>MILSDKDIIDYVTSKRIIIKPFNKDFVGPCSYDVTLGDEFIIYDDEVYDLSKELNYKRIKIKNSILVCPLNYNLTEEKINYFKEKYNVDYVVEGGVLGTTNEYIELPNDISAQYQGRSSLGRVFLTSHQTAG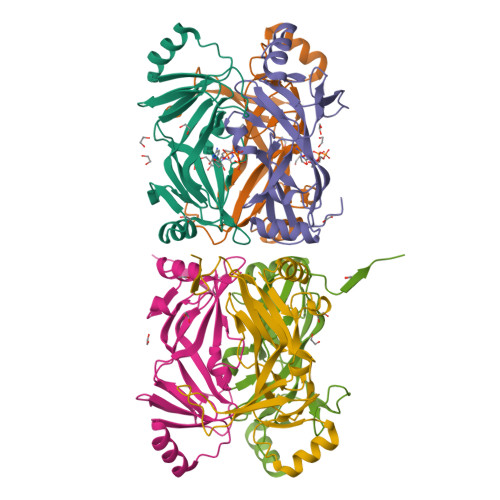WIDAGFKGKITLEIVAFDKPVILYKNQRIGQLIFSKLLSPADVGYSERKTSKYAYQKSVMPSLIHLDNHKKD[2x]> MDVDSDVNVSRLRDELHKVANEETDTATFNDDAPSGATCRICRGEATEDNPLFHPCKCRGSIKYMHESCLLEWVASKNIDISKPGADVKCDICHYPIQFKTIYAENMPEKIPFSLLLSKSILTFFEKARLALTIGLAAVLYIIGVPLVWNMFGKLYTMMLDGSSPYPGDFLKSLIYGYDQSATPELTTRAIFYQLLQNHSFTSLQFIMIVILHIALYFQYDMIVREDVFSKMVFHKIGPRLSPKDLKSRLKERFPMMDDRMVEYLAREMRAHDENRQEQGHDRLNMPAAAADNNNNVINPRNDNVPPQDPNDHRNFENLRHVDELDHDEATEEHENNDSDNSLPSGDDSSRILPGSSSDNEEDEEAEGQQQQQQPEEEADYRDHIEPNPIDMWANRRAQNEFDDLIAAQQNAINRPNAPVFIPPPAQNRAGNVDQDEQDFGAAVGVPPAQANPDDQGQGPLVINLKLKLLNVIAYFIIAVVFTAIYLAISYLFPTFIGFGLLKIYFGIFKVILRGLCHLYYLSGAHIAYNGLTKLVPKVDVAMSWISDHLIHDIIYLYNGYTENTMKHSIFIRALPALTTYLTSVSIVCASSNLVSRGYGRENGMSNPTRRLIFQILFALKCTFKVFTLFFIELAGFPILAGVMLDFSLFCPILASNSRMLWVPSICAIWPPFSLFVYWTIGTLYMYWFAKYIGMIRKNIIRPGVLFFIRSPEDPNIKILHDSLIHPMSIQLSRLCLSMFIYAIFIVLGFGFHTRIFFPFMLKSNLLSVPEAYKPTSIISWKFNTILLTLYFTKRILESSSYVKPLLERYWKTIFKLCSRKLRLSSFILGKDTPTERGHIVYRNLFYKYIAAKNAEWSNQELFTKPKTLEQAEELFGQVRDVHAYFVPDGVLMRVPSSDIVSRNYVQTMFVPVTKDDKLLKPLDLERIKERNKRAAGEFGYLDEQNTEYDQYYIVYVPPDFRLRYMTLLGLVWLFASILMLGVTFISQALINFVCSFGFLPVVKLLLGERNKVYVAWKELSDISYSYLNIYYVCVGSVCLSKIAKDILHFTEGQNTLDEHAVDENEVEEVEHDIPERDINNAPVNNINNVEEGQGIFMAIFNSIFDSMLVKYNLMVFIAIMIAVIRTMVSWVVLTDGILACYNYLTIRVFGNSSYTIGNSKWFKYDESLLFVVWIISSMVNFGTGYKSLKLFFRNRNTSKLNFLKTMALELFKQGFLHMVIYVLPIIILSLVFLRDVSTKQIIDISHGSRSFTLSLNESFPTWTRMQDIYFGLLIALESFTFFFQATVLFIQWFKSTVQNVKDEVYTKGRALENLPDES

Doa10 (MARCHF6 in metazoans) is a large polytopic membrane-embedded E3 ubiquitin ligase in the endoplasmic reticulum (ER) that plays an important role in quality control of cytosolic and ER proteins. Overall, the TMD of Doa10 can be divided into the three subregions: the N-terminal domain (NTD), the middle domain, and the C-terminal domain (CTD), which are formed by TMs 1–4, 5–10, and 11–14, respectively. Our study reveals how extended hydrophobic sequences at the termini of substrate proteins are recognized by Doa10 as a signal for quality control.

Single particle cryo-EM analysis of purified Doa10 yielded only one major class, which could be refined to a three-dimensional (3D) reconstruction at 3.2-Å overall resolution. We also note that the N-terminal RING-CH domain (residues 1–113) and the loop between TMs 2 and 3 (L2/3; residues 242–463) are only visible at low resolution due to high conformational heterogeneity. Our study reveals the highly unusual architecture of Doa10, where its TMD is arranged in a C-shape architecture with its central cavity filled with lipids. In our cryo-EM map, this cavity is filled with detergent and lipid molecules, suggesting that it would be occupied with lipids in the native membrane. As a result, the TMD itself contains two sizable intra-TMD cavities each surrounded by TMs 1–5 (cavity 1) and by TMs 5–10 (cavity 2), respectively, and both are partly continuous from the central cavity. Our cryo-EM structure shows that both cavities are occupied by lipids. Interestingly, cavity 2 is occupied with a triglyceride in addition to a phospholipid. The conserved middle domain of Doa10 forms a lateral tunnel-like cavity, the entrance of which faces the central cavity and is open to the cytosol. However, the tunnel interior seems water-filled as the cavity is lined by a mixture of polar, charged, and hydrophobic amino acids. Consistent with this, we also observed in the MD simulations that the tunnel interior is filled with many water molecules. On the other hand, the back of the tunnel seems at least partially blocked by a phospholipid in our cryo-EM structure (PC4 in Fig. 2a, b).> X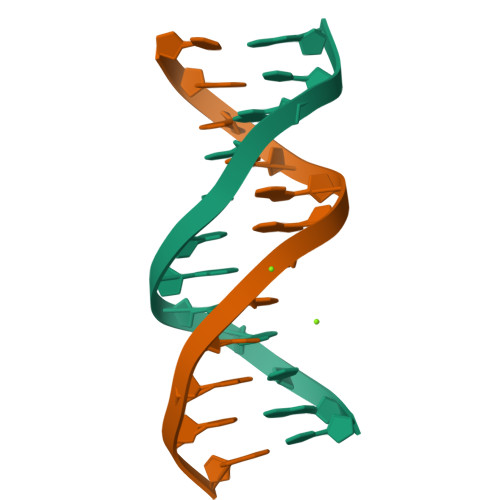RRRR>[2x]MGISWLDIYHVVSATVPLYVSMTLGFLSARHLKLFSPEQCAGINKFVAKFSIPLLSFQIISENNPFKMSPKLILSDILQKFLVVVVLAMVLRFWHPTGGRGGKLGWVITGLSISVLPNTLILGMPILSAIYGDEAASILEQIVVLQSLIWYTILLFLFELNAARALPSSGASLEHT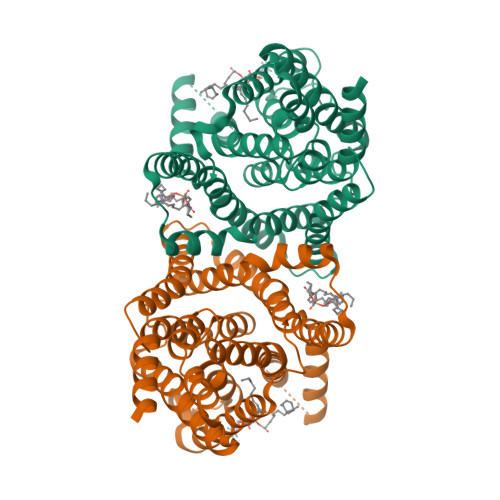GNDQEEANIEDEPKEEEDEEEVAIVRTRSVGTMKILLKAWRKLIINPNTYATLIGIIWATLHFRLGWNLPEMIDKSIHLLSDGGLGMAMFSLGLFMASQSSIIACGTKMAIITMLLKFVLGPALMIASAYCIRLKSTLFKVAILQAALPQGVVPFVFAKEYNLHPEIISTGVIFGMLIALPTTLAYYFLLDLPGENLYFQ Virus ΦcrAss001 (Kehishuvirus primarius) was the first representative of this order to be isolated in pure culture from human faecal samples. Here, we present the characterization of ΦcrAss001 using cryo-electron microscopy (cryo-EM), enabling de novo structure building and elucidation of functions for around 1,440 protein subunits constituting the virion, leading to the identification of a novel ‘crass fold’ in the distal part of the tail. The virion possesses a short non-contractile tail extending approximately 44 nm from an icosahedral capsid. The extended tail barrel formed by widely conserved paralogous ring proteins has a high capacity for storage of cargo proteins alongside the capsid cargo zone, ensuring that the proteins required for the initial stages of crassvirus infection are carried inside virions and delivered to the host cell.

The portal protein is considered the nucleation point for capsid assembly and serves as the docking site for the tail. The portal is surrounded by the five-fold symmetric capsid vertex, contacting 10 major capsid protein subunits. The surrounding capsid vertex was also reconstructed with C5-symmetrical averaging to a resolution of 3.30 Å. The portal oligomer positioned in the vertex occludes the binding site of the capsid auxiliary protein gp36, which is substituted by two copies of the portal vertex specific auxiliary protein, gp57. The gp57 dimer has approximate two-fold symmetry, reinforced by disulfide bonds between residues 47–47 and 25–88 of the two subunits. Notably, hexameric capsomers bordering the unique vertex contain trimer capsid fibres of gp21, in contrast to the hexamers bordering other pentameric vertices, which contain dimeric capsid fibres of gp29.

>[6x]MAGKLGKFQMLGFQHWKGLTSDNHLGAIFQQAPQKATNLMVQLLAFYRGKSLDTFLNSFPTREFEDDNEYYWDVIGSSRRNIPLVEARDENGVVVAANAANVGVGTSPFYLVFPEDWFADGEVIVGNLNQVYPFRILGDARMEGTNAVYKVELMGGNTQGVPAERLQQGERFSIEFAPVEKELSRKVGDVRFTSPVSMRNEWTTIRIQHKVAGNKLNKKLAMGIPMVRNLESGKQVKDTANMWMHYVDWEVELQFDEYKNNAMAWGTSNRNLNGEYMNFGKSGNAIKTGAGIFEQTEVANTMYYNTFSLKLLEDALYELSASKLAMDDRLFVIKTGERGAIQFHKEVLKTVSGWTTFVLDNNSTRVVEKVQSRLHSNALSAGFQFVEYKAPNGVRVRLDVDPFYDDPVRNKILHPMGGVAFSYRYDIWYIGTMDQPNIFKCKIKGDNEYRGYQWGIRNPFTGQKGNPYMSFDEDSAVIHRMATLGVCVLDPTRTMSLIPAILQG;>[5x]MVISINQVRQLYVAKALKANTAALTTAGDIVPKADTAKTTLYFQSMSPAGIVASDKINLKHVLYAKATPSEALAHKLVRYSVTLDADVSATPVAGQNYILRLAFRQYIGLSEEDQYFKYGEVIARSGMTASDFYKKMAISLAKNLENKTESTPLVNIYLISAAAASTDVPVTSATKESDLTATDYNQIIIEETEQPWVLGMMPQAFIPFTPQFLTITVDGEDRLWGVATVVTPTKTVPDGHLIADLEYFCMGARGDIYRGMGYPNIIKTTYLVDPGAVYDVLDIHYFYTGSNESVQKSEKTITLVAVDDGSHTAMNALIGAINTASGLTIATL;>MAGQQGIYCAPDNIVPNRDRVDVGCAPDGAMQLWVMEYEVTGIGKGCAMCKAINPQQAEMLLKSNGIYNGSSYLYKVTRIEQVIVPPCNGLMAEQVVTYKDVVS[2x];>MKTLRTLKISPNAPDINSVWLYKGTMKYFNNGEWETIGGESEPYVLPAATTSTIGGVKKATNVGNLATGAELATVVTKVNAILSALKVADIMVEDAN[3x];>MADFLNFPRQMLPFSKKTKQWRKDCLLWANQKTFFNYSLVRKSVIHKKINYDLLNGRLHMSDLELVLNPDGIKAAYIPDRLQHYPIMNSKLNVLRGEESKRVFDFKVVVTNPNAISEIEDNKKNELLQRLQEMITDTSISEDEYNIKLEKLNDYYTYEWQDIREVRANELLNHYIKEYDIPLIFNNGFMDAMTCGEEIYQCDIVGGEPVIERVNPLKIRIFKSGYSNKVEDADMIILEDYWSPGRVIDTYYDVLSPKDIKYIETMPDYIGQGAVDQMDNIDERYGFVNQNMIGDEITVRDGTYFFDPANLFTEGIANSLLPYDLAGNLRVLRLYWKSKRKILKVKSYDPETGEEEWNFYPENYVVNKEAGEEVQSFWVNEAWEGTMIGNEIFVNMRPRLIQYNRLNNPSRCHFGIVGSIYNLNDSRPFSLVDMMKPYNYLYDAIHDRLNKAIASNWGSILELDLSKVPKGWDVGKWMYYARVNHIAVIDSFKEGTIGASTGKLAGALNNAGKGMIETNIGNYIQQQINLLEFIKMEMADVAGISKQREGQISQRETVGGVERATLQSSHITEWLFTIHDDVKKRALECFLETAKVALKGRNKKFQYILSDTSTRVMEIDGDEFAEADYGLVVDNSNGTQELQQKLDTLAQAALQTQTLSFSTITKLYTSSSLAEKQRLIEKDEKQIRERQAQAQKEQLEAQQQIAAMQQQQKEAELLQKEEANIRDNQTKIIIAQIQSEGGPDEEDGIMIDDYSPEAKANLAEKIREFDEKLKLDKDKLKLDKKKAETDASIKRQALRKKSSTTNK[2x]> MDTETWAAAARPSRDALINRITHQIRQSLELDQILRATVEEVRAFLGTDRVKVYRFDPEGHGTVVAEARGGERLPSLLGLTFPAGDIPEEARRLFRLAQVRVIVDVEAQSRSISQPESWGLSARVPLGEPLQRPVDPCHVHYLKSMGVASSLVVPLMHHQELWGLLVSHHAEPRPYSQEELQVVQLLADQVSIAIAQAELLEQARQKAQQERLINQIAALVYSPLHPETTLTTVLEQLAAGLQGIGARLRIHFMGADTLCCHGVQPPASYDTWLQEQLGRAGGAGGWVKMWSLSHLEKWPELQEQMKQTPIRGLLVAQLAWNDQPVGWLSVFRGAVYQETHWAGYRWFTQGDPRQELPLISFAAWRELKIDEPKAWSAAEQELMSRVGVHLALSITQNQLYRQLQTLNARLEQEVQERTAASLHHHHHH

One major class in microorganisms and plants is the phytochromes (Phys), a diverse collection of dimeric chromoproteins that employ a covalently-bound bilin (or open chain tetrapyrrole) prosthetic group that can assume two conformers, a red light-absorbing Pr state and a metastable far-red light-absorbing Pfr state. Through fast photointerconversion between Pr and Pfr and slower thermal reversion of Pfr back to Pr, Phys acts as photoswitches in detecting light fluence, duration, photoperiod, and the ratio of red and far-red light. The bilin is buried within a GAF domain pocket, which through numerous chromophore/protein contacts provides the unique absorption and photochromicity of these photoreceptors. Besides canonical Phys, cyanobacteria express several variants, including a PAS-less subfamily that harbors just the GAF and PHY domains for light detection.

Here, we began to address this controversy by generating an X-ray crystallographic structure of SyB-Cph1 as Pr, in this case using the full PSM encompassing both the GAF and PHY domains and the connecting hairpin. This fragment assembled as a head-to-head dimer consistent with other bacterial Phys but included a unique GAF domain dimerization contact involving a 15-residue sequence previously defined as the Arg-Ile-Thr (RIT) motif that is conserved among PAS-less Phys, and relatively straight and parallel α-helical spines uncharacteristic of most microbial Phy structures. Surprisingly, our PSM structure also revealed a unique hybrid architecture that included a dark-adapted chromophore in a ZZZssa configuration typically seen for Pr but partially rotated to a “Pfr-like” position within the binding pocket along with an α-helical hairpin typically seen for Pfr. PCB was connected to the GAF domain by a thioether linkage between the C31 carbon of the ethylidene side chain of PCB and the sulfur moiety of Cys138, and was buried within the GAF domain in the expected ZZZssa conformation for Pr. As with canonical Phys, the pyrroles of rings A-C along with an adjacent histidine imidazole group (His139) and the main chain carbonyl of Asp86 fixed a central water (designated pyrrole water), which participates in proton release and uptake during photoconversion. The electron density map of the hairpin region easily identified one strand of the loop as α-helical, and like the Pfr state in other Phys (e.g., (10, 20, 26)), employed a serine (Ser361) in the hairpin to contact the GAF domain via Asp86 within the Asp-Ile-Pro (DIP) sequence close to the chromophore. Superpositions based on the GAF domains comparing the bilin position of SyB-Cph1(GAF-PHY) to those in the Pr models of Synechocystis (Syn) Cph1 (25) and Syn-Cph2 (20) and the Pfr model of the bathyPhy from Pseudomonas aeruginosa (Pa-BphP), showed that the GAF domains and the A-pyrrole ring positions aligned well despite photostate differences.> EVSQDLFNQFNLFAQYSAAAYCGKNNDAPAGTNITCTGNACPEVEKADATFLYSFEDSGVGDVTGFLALDNTNKLIVLSFRGSRSIENWIGNLNFDLKEINDICSGCRGHDGFTSSWRSVADTLRQKVEDAVREHPDYRVVFTGHSLGGALATVAGADLRGNGYDIDVFSYGAPRVGNRAFAEFLTVQTGGTLYRI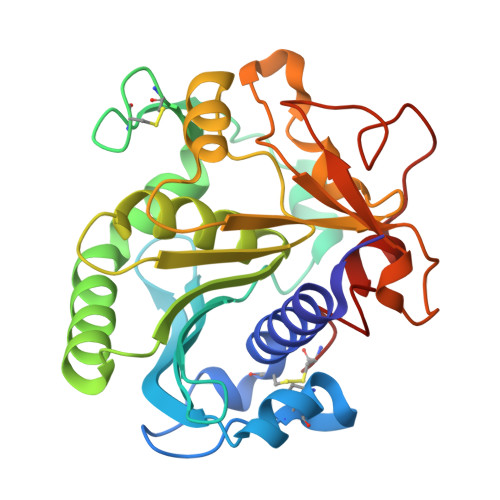THTNDIVPRLPPREFGYSHSSPEYWIKSGTLVPVTRNDIVKIEGIDATGGNNQPNIPDIPAHLWYFGLIGTCL>TCGGCGCCGA[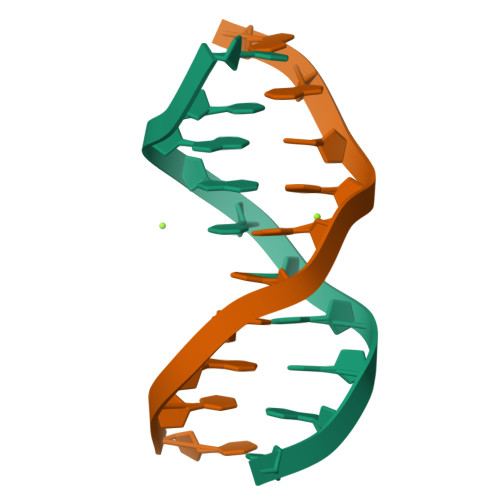6x]> EPIRYAIPEELDRGSLVGNLAKDLGFGVGDLPTRNLRVIAEKKFFTVSPENGNLLVSDRIDREEICGKKSTCVLEFEMVAEKPLNFFHVTVLIQDINDNPPTFSQNITELEISELALTGATFALESAQDPDVGVNSLQQYYLSPDPHFSLIQKENLDGSRYPELVLKAPLDREEQPHHHLVLTAVDGGEPSRSCTTQIRVIVADANDNPPVFTQDMYRVNVAENLPAGSSVLKVMAIDMDEGINAEIIYAFINIGKEVRQLFKLDSKTGELTTIGELDFEERDSYTIGVEAKDGGHHTAYCKVQIDISDENDNAPEITLA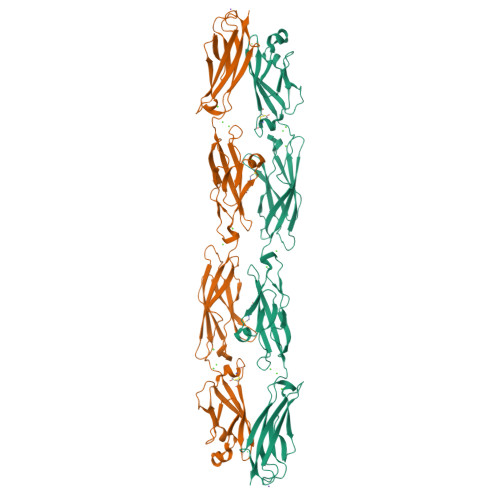SESQHIQEDAELGTAVALIKTHDLDSGFNGEILCQLKGNFPFKIVQDTKNTYRLVTDGALDREQIPEYNVTITATDKGNPPLSSSKTITLHILD>[32x]XSKLLELLRKLL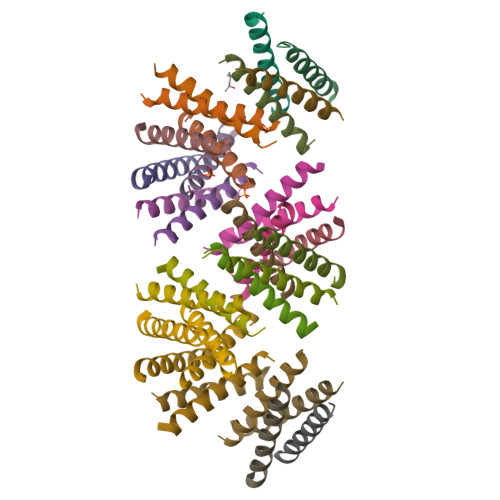EALHKAIELLEKWGX DMHBI+ | C22 H26 N3 O4 | 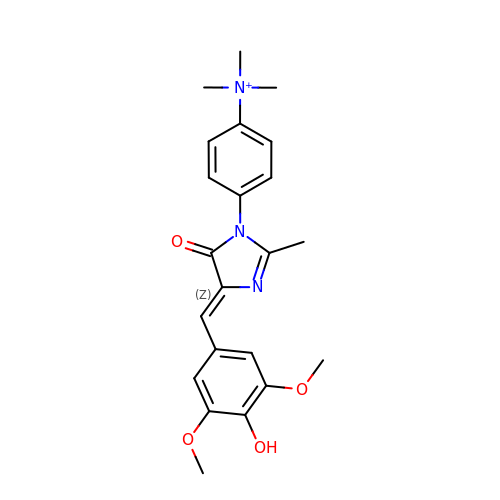SMSBZPALSUJZFM-UHFFFAOYSA-O> LSLLSDGIDEEELIEAADFQGLYAEVKACSSELESLEMELRQQILVNIGKILQDQPSMEALEASLGQGLCSGGQVEPLDGPAGCILECLVL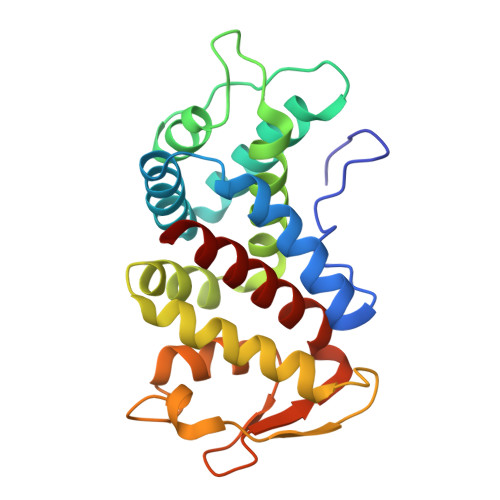DSGELVPELAAPIFYLLGALAVLSETQQQLLAKALETTVLSKQLELVKHVLEQSTPWQEQSSVSLPTVLLGDCWDEKNPTWVLLEECGLRLQVESPQVHWEPTSLIPTSALYASLFLLSSLGQ> AMRQCAIYGKGGIGKSTTTQNLVAALAEMGKKVMIVGCDPKADSTRLILHSKAQNTIMEMAAEAGTVEDLELEDVLKAGYGGVKCVESG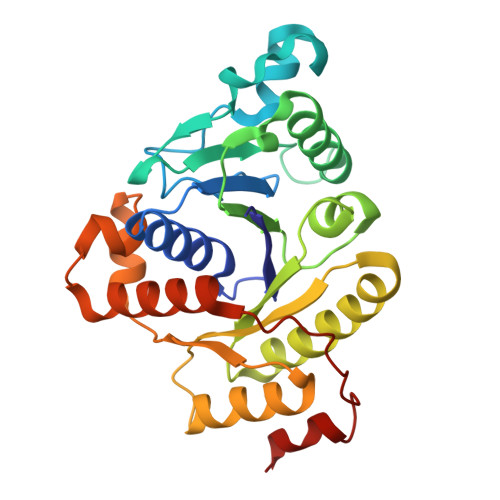GPEPGVGCAGRGVITAINFLEEEGAYEDDLDFVFYDVLGDVVCGGFAMPIRENKAQEIYIVCSGEMMAMYAANNISKGIVKYANSGSVRLGGLICNSRNTDREDELIIALANKLGTQMIHFVPRDNVVQRAEIRRMTVIEYDPKAKQADEYRALARKVVDNKLLVIPNPITMDELEELLMEFG>[12x]MLYTDSLNYKQLSTVSDDMQSYLPVAKEIAKIAQGGHELDPEDYLLIRDEESPGVTKKRIEKFAPENYLGAAIRLQRVLQKSGVLEIKSDSLPGDLTVWESFFNKVDKRNSSLKDFVIDVFTEALVNKYCYVQVELSKLDFDTVTEAEAEGILSTRKPYYFKIPLQSIMVEKCDGDTIQWIKYKRLDKIDNPFDKTIYNMSYVLIDDQHITTWTYYDIIVSDSGGISKIWDQSLNYGKGAYRSIDKEKDKADPVSFAHNRGSCPVVRYRMDESLYMADQVYLAQRMIYGLSMNLFHTAANAGFVQKWIRPYIAGNDTRISKESGGASYIPLPKEALNEIIKKYAESLGDESVIMADFFTFEELAGTSVEMQIGLIERLRNYIFTAILFNNAKFEQSTSDSQSGAAKEIDFYVQNLALKDHGSGIVEFTRSLLHHTAKAFGYDSGGSIVVSGMDRYDVRPIEQVLSLIERLFKLPQLAIPKDLLIESMSQLSRLIIENTTFEYKNTLNDAIISNIDEYLNSVKKQSNDAFNETVK

A-1(L) is a Myoviridae cyanophage isolated in 1970s9 that specifically infects the model cyanobacterium Anabaena sp. PCC 7120. Using cryo-electron microscopy (cryo-EM), we solved the structure of A-1(L) tail machine, which consists of three parts: a 205-Å-long neck, a 1045-Å-long contractile tail with a complicated baseplate, and six pairs of tail fibers. The dodecameric gp2 portal, the pentadecameric gp5 and the hexameric gp7 sequentially constitute the neck of A-1(L), to which five neck fibers are attached. The long and contractile tail of A-1(L) contains 24 rings of gp10 hexamers that form the tube, surrounded by the sheath of 24 helically stacked gp9 hexamers.

Twelve gp2 subunits form a dodecameric portal with a central channel of 25 Å in diameter at the narrowest tunnel loop. Notably, we observed two extra densities: one in the central channel and one around the wing of portal dodecamer, which were assigned to two segments of the dsDNA genome in our model, respectively. The dodecameric portal is surrounded by five major capsid gp4 hexamers in a 12:5 symmetry-mismatch pattern. The wing domain (residues Met1-Tyr275) of portal interacts with the A domain (residues Ser178-Asn282, Leu353-Gln365) and P domain (residues Asn22-Arg177, Leu283-Asp352) of corresponding major capsid subunit, forming a circular cleft that accommodates a segment of the genomic dsDNA. The dodecameric portal/gp2 forms a channel for the passage of genomic DNA, whereas the hexameric neck/gp7 provides an interface for the docking of tail. At the 5-fold vertex of A-1(L) capsid, the 12-fold portal/gp2 dodecamer, the 15-fold neck/gp5 pentadecamer, and the 6-fold neck/gp7 hexamer are sequentially interlocked to form a symmetry-mismatched neck. The dodecameric portal/gp2, gp5 pentadecamer and gp7 hexamer form a symmetry-mismatched neck, which are perfectly accommodated to the 5-fold vertex of icosahedral capsid.> MDDLFEVFEEQPRAQKKRKASPDVEMADGAAAAAPVANAAAAVTHPQAQAAPAPQKDNIDNNDNNNNNTTTSAVQPTIPNGDAAAAADDVQSPQSPHGLGDNKRRKKTDEAEPIMTDAFQTAESREVTGAQGFAPTEGESIVLSHNIQHQVALPPDLDYEYIPLSEHKPPAEPARTYSFKLDPFQALSVASIEREESVLVSAHTSAGKTVVAEYAIAQCLKKNQRVIYTSPIKALSNQKYRDFQAEFGDVGLMTGDVTINPTASCLVMTTEILRSMLYRGSEIMREVAWVVFDEIHYMRDKIRGVVWEETIILLPDKVRYVFLSATIPNAFQFAEWIAKIHRQACHVVYTDFRPTPLQNYFFPAGGKGILLIVDEKGNFKENNFNQAMAMIEEKKGTDSNDWSAKQKGKGKNKKTNKGGEAADEKADIAKIIKMILKKNFQPVIVFNFSKRECEQMALASSSMKFNAPDEENMVNK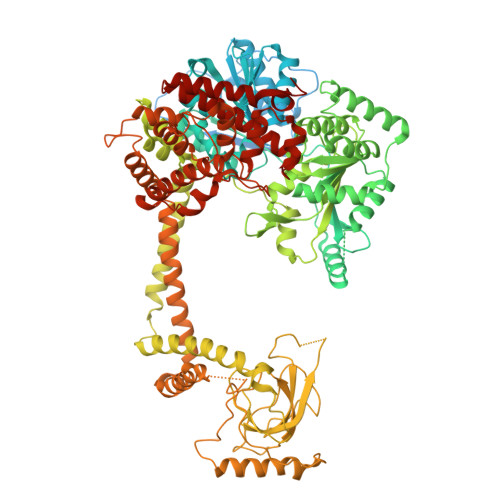VFENALASLSEDDKNLPQISNILPLLRKGIGVHHSGLLPILKETIEILFQEGLIKVLFATETFSIGLNMPARTVVFTQVTKWDGQQRRPLTSSEYIQMAGRAGRRGLDDRGIVIMMVDDKLEPETARAIVVGNQDKLNSAFHLGYNMVLNLLRIEAISPEYMLERCFFQFQNAASVPQLERELISLQQERDAIIIPDESIVKDYYGVRQQLEEYNKDMVFVIQHPQNCLGFFQEGRLIHIKSPSGVDYGWGVLIKHIQRQTPKNGQPPYPEQESYVLDVLLKVSGDFNPKTRGEGPMPEGIMPAGKDSKNARWEVVPCLLNCLRALGQLRVFLPKRLESADEKDGVGKAVDEISRRFPDGIPILDPMENMGINDDSFKKLLRKIEVLESRLVANPLHNSPLLVELWNQYSLKMQLGEQIKEKKKAIARAHSVAQLDELKSRKRVLRRLGFINDAEVVQMKARVACEISSTEGHELLLAELLFNRFFNELSPEICACILSCFIFDEKIETQALKEELAKPFREIQAQARIIAKVSAESKLDVNEDEYVQSLKWQLMETVLAWAQGRPFSEICKMTNVYEGSLIRLFRRLEELLRQMAEAARVMGSEELKDKFELSLSKIRRDIVSFNSLYL> MQYDDDCKLARGGPPATIVAIDEESRNGTILVDNMLIKGTAGGPDPTIELSLKDNVDYWVLLDPVKQMLFLNSTGRVLDRDPPMNIHSIVVQVQCVNKK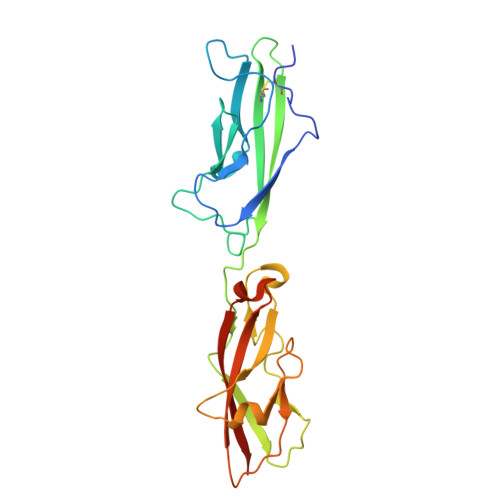VGTVIYHEVRIVVRDRNDNSPTFKHESYYATVNELTPVGTTIFTGFSGDNGATDIDDGPNGQIEYVIQYNPEDPTSNDTFEIPLMLTGNVVLRKRLNYEDKTRYYVIIQANDRAQNLNERRTTTTTLTVDLEHHHHHH> MGRGKVKPNRKSTGDNSNVVTMIRAGSYPKVNPTPTWVRAIPFEVSVQSGIAFKVPVGSLFSANFRTDS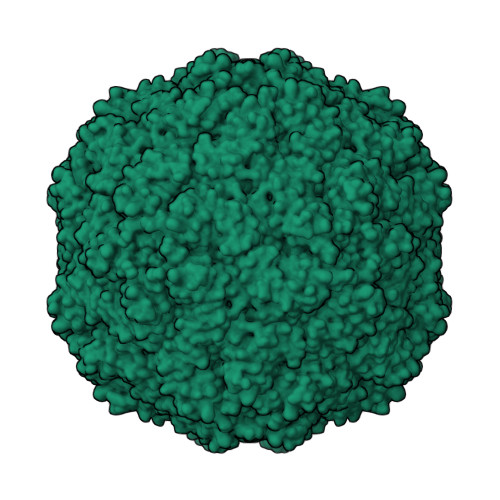FTSVTVMSVRAWTQLTPPVNEYSFVRLKPLFKTGDSTEEFEGRASNINTRASVGYRIPTNLRQNTVAADNVCEVRSNCRQVALVISCCFN> GTERKLLERSRRLQEESKRLLD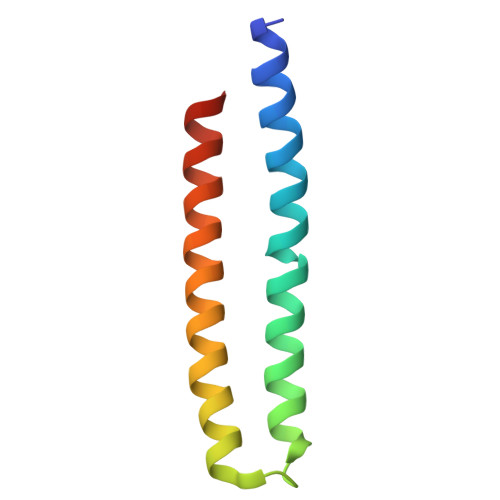EMAEIMRRIKKLLKKARGADEKVLDELRKIIERIRELLDRSRKIHERSEEIAYKEE> EVPTWHRLSSYR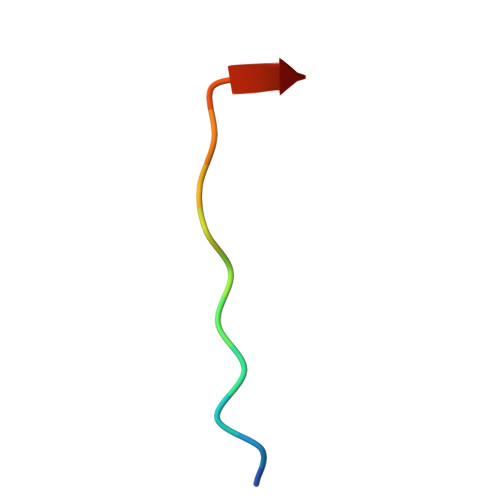G> KTSDANETEDHLESLICKVGEKSACSLESNLEGLAGVLEADLPNYKSKILRLLCTVARLLPEKLTIYTTLVGLLNARNYNFGGEFVEAMIRQLKESLKANNYNEAVYLVRFLSDLVNCHVIAAPSMVAMFENFVSVTQEEDVPQVRRDWYVYAFLSSLPWVGKEL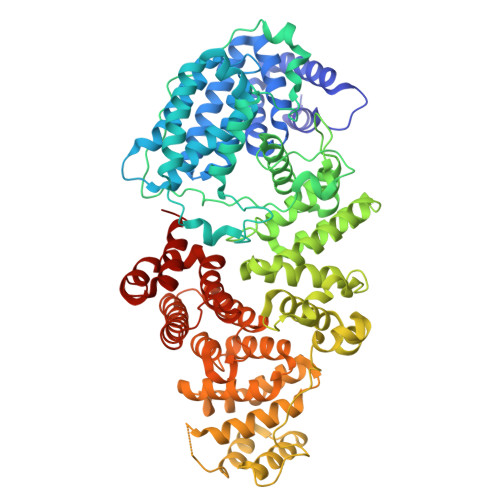YEKKDAEMDRIFANTESYLKRRQKTHVPMLQVWTADKPHPQEEYLDCLWAQIQKLKKDRWQERHILRPYLAFDSILCEALQHNLPPFTPPPHTEDSVYPMPRVIFRMFDYTDDPEGPVMPGSHSVERFVIEENLHCIIKSHWKERKTCAAQLVSYPGKNKIPLNYHIVEVIFAELFQLPAPPHIDVMYTTLLIELCKLQPGSLPQVLAQATEMLYMRLDTMNTTCVDRFINWFSHHLSNFQFRWSWEDWSDCLSQDPESPKPKFVREVLEKCMRLSYHQRILDIVPPTFSALCPSNPTCIYKYGDESSNSLPGHSVALCLAVAFKSKATNDEIFSILKDVPNPNQDDDDDEGFSFNPLKIEVFVQTLLHLAAKSFSHSFSALAKFHEVFKTLAESDEGKLHVLRVMFEVWRNHPQMIAVLVDKMIRTQIVDCAAVANWIFSSELSRDFTRLFVWEILHSTIRKMNKHVGAQSEQKNLFLVIFQRFIMILTEHLVRCETDGTSVLTPWYKNCIERLQQIFLQHHQIIQQYMVTLENLLFTAELDPHILAVFQQFCALQA> MLKKVLVGMFGAALIAGIGMTTAQAYDVK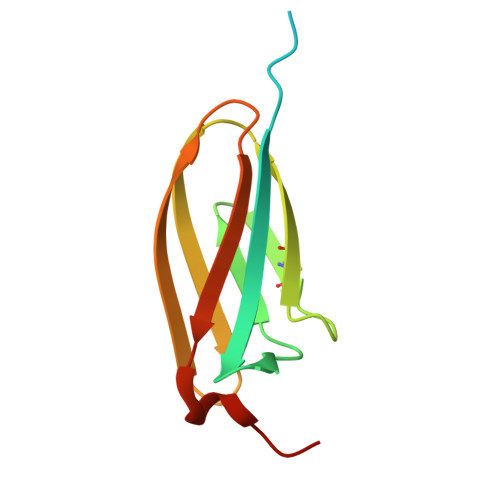PAKLWVTAIAIGTPIVGAEIKVGDEECTTGNNGTCVFELRPGTYAISVHEHGGQSAHKEVSLEEGNILFVSLDLGAKARHPSGSH> GPLHMVKVALAGCPNVGKTSLFNALTGTKQYVANWPGVTVEKKEGVFTYKGYTINL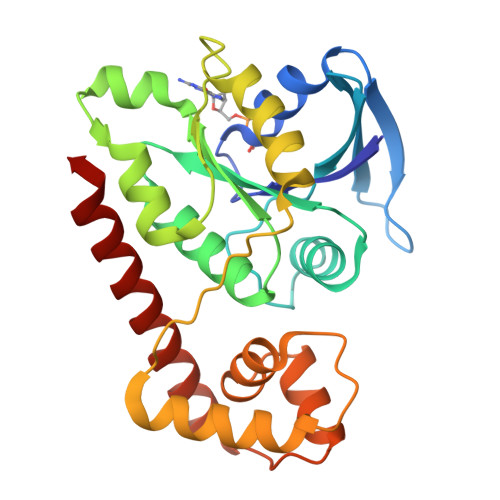IDLPGTYSLGYSSIDEKIARDYLLKGDADLVILVADSVNPEQSLYLLLEILEMEKKVILAMTAIDEAKKTGMKIDRYELQKHLGIPVVFTSSVTGEGLEELKEKIVEYAQKNTILHRMILDYGEKVESEIKKVENFLRDKKLRINPRYFALKYLSGDPEFYSEGVKLGLPELSEEERIGYRLLIAKRKREYVENVVKEAFAD> GEFTQSVSRLQSIVAGLKNAPSDQLINIFESCVRNPVENIMKILKGIGETFCQHYTQSTDEQPGSHIDFAVNRLKLAEILYYKILETVMVQETRRLHGMDMSVLLEQDIFHRSLMACCLEIVLFAYSSPRTFPWIIEVLNLQPFYFYKVIEVVIRSEEGLSRDMVKHLNSIEEQILESLAWSHDSAL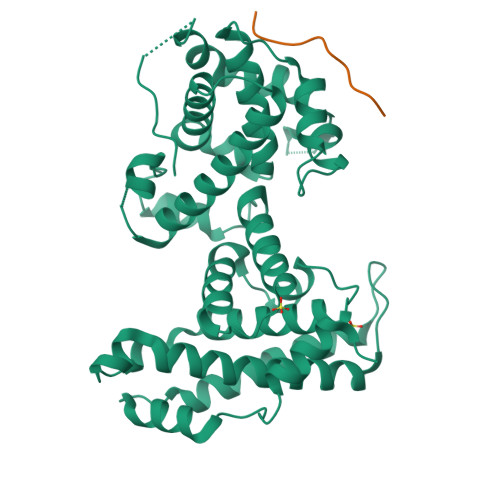WEALQVSANKVPTCEEVIFPNNFETGNNRPKRTGSLALFYRKVYHLASVRLRDLCLKLDVSNELRRKIWTCFEFTLVHCPDLMKDRHLDQLLLCAFYIMAKVTKEERTFQEIMKSYRNQPQANSHVYRSVLLKSIKEERGDLIKFYNTIYVGRVKSFALKYDLANQDHMMDAPPLSPFPHIKQQ;> RIACEEEFSD> GSVEEIRLP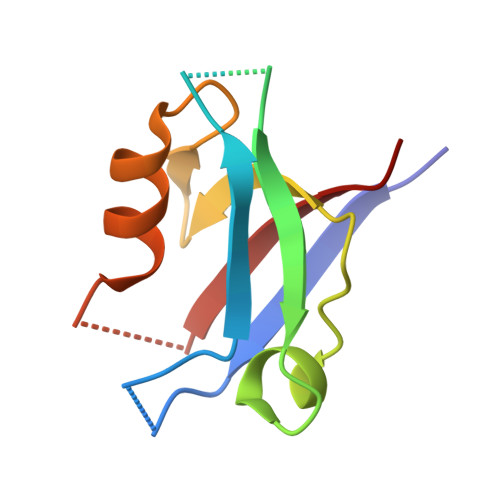RAGGPLGLSIVGGSDHSSHPFGVQEPGVFISKVLPRGLAARSGLRVGDRILAVNGQDVRDATHQEAVSALLRPCLELSLLVRRD> MTARIALASLFVVAAVLAQPWQTTTQRWVLGVSIAAVIVLLAWWKGMFLTTRIGRALAMVRRNR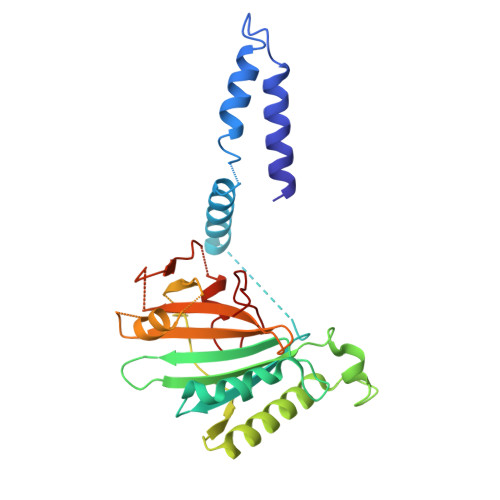AEDTVETDAHRATVVLRVDPAAPAQLPVVVGYLDRYGITCDKVRITHRDAGGTRRSWISLTVDAVDNLAALQARSARIPLQDTTEVVGRRLADHLREQGWTVTVVEGVDTPLPVSGKETWRGVADDAGVVAAYRVKVDDRLDEVLAEIGHLPAEETWTALEFTGSPAEPLLTVCAAVRTSDRPAAKAPLAGLTPARGRHRPALAALNPLSTERLDGTAVPL> MVPISPIETVPVKLKPGMDGPKVKQWPLTEEKIKALVEICTEMEKEGKISKIGPENPYN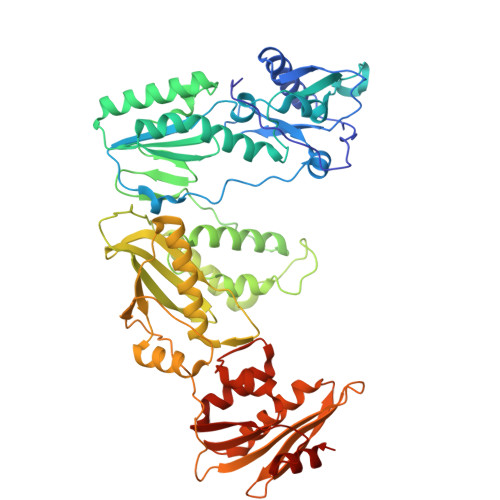TPVFAIKKKDSTKWRKLVDFRELNKRTQDFWEVQLGIPHPAGLKQKKSVTVLDVGDAFYSVPLDKDFRKYTAFTIPSINNETPGIRYQYNVLPMGWKGSPAIFQSSMTKILEPFRKQNPDIVIYQYVDDLYVGSDLEIGQHRTKIEELRQHLLRWGFTTPDKKHQKEPPFLWMGYELHPDKWTVQPIVLPEKDSWTVNDIQKLVGKLNWASQIYAGIKVRQLSKLLRGTKALTEVVPLTEEAELELAENREILKEPVHGVYYDPSKDLIAEIQKQGQGQWTYQIYQEPFKNLKTGKYARMKGAHTNDVKQLTEAVQKIATESIVIWGKTPKFKLPIQKETWEAWWTEYWQATWIPEWEFVNTPPLVKLWYQLEKEPIIGAETFYVDGAANRETKLGKAGYVTDRGRQKVVPLTDTTNQKTELQAIHLALQDSGLEVNIVTDSQYALGIIQAQPDKSESELVSQIIEQLIKKEKVYLAWVPAHKGIGGNEQVDKLVSAG>SGGGDGSTYSAEIRRTTMGVPHIKAGNWGSAGYGFGYVQAQDNLCTMADSFLTYRGERSRHLGGSAQLVYNSTLGRPRNIDSDFFHRHVISDEAVDRTMAAQPAKLLQMVEGFAAGYNRYVREAKAGGSAHAACRSEAWVQPITARDVWRRIYAANLAGGYSNFAEAIANAQPPQAKAGAQEPAAFEPGRTRAPSLQGSNMYGFGTAATGEGSGVLFGNPHWYWKGPDRFYQAQLTIDGEANVSGVSFLGLPVIQIGFNDSVAWSHTVSTARRFGFFQLSLVQGEPTSYLRDGVPVKMKPATITVPSRNADGSVSDVTRTLYHSEFGPLVNLAGLNPALAWSQGTAFAIRDINGENFRTLRTWMRWNQAKSLDEFIAIQKEEASIPWVNTVAVGRGSAKAWYADIGAVPNVSPAQTAACTTPFGMAVGQALPNVPFFDGSRSECDWLTDADSVQKGAVGVSRMPSLQRDDYVGNMNDSYWLANVHAPLTGYPAIFGPAGTSAQTLRTRMGHTMALERLAGTDGYAGNKATSAVVREMVLGSRVFSAERFKDEVLDLICTPAQWTVNGAAVDAAQACAVLAAWDNRGRKDSRGSHLWDEFWSRVPTASLFTVPFSAADPL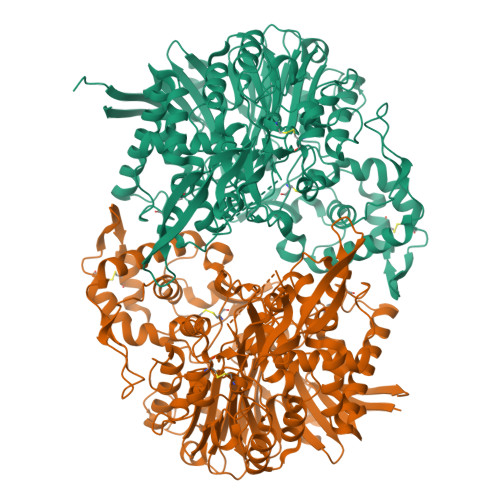NTPRGINAAAADALRQAMATAIARVGQSGYALDAPRGEVLYATRGGTRLPLYGGCGAMGYFTITCSENDITQGGYSMDGQPNASNSYMQVVSFPASGVQAHTFLTFSLSDDPASPHHGDYTKAYSAGQWLRVPFTEAEITGNADYRTATVKELEHHHHHH[4x]> GGUUGCCGAAUCCUUUACUUGGUACGGAGGAACCGCUUUUUGGGGUUAAUCUGCAGUGAAGC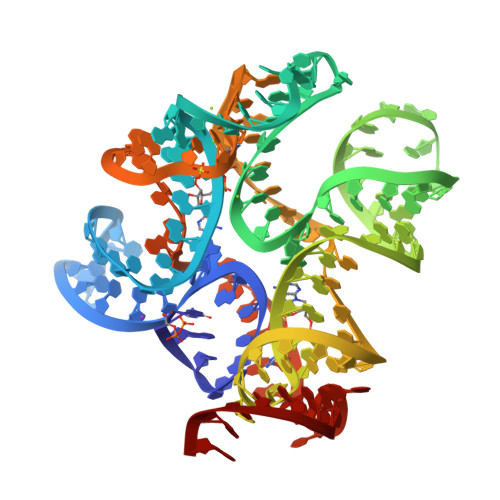UGCAGUAGGGAUACCUUCUGUCCCGCACCCGACAGCUAACUCCGGAGGCAAUAAAGGAAGGAG>GTDDATADSRKTYTLTDYLKNTYRLKLYSLRWISDHEYLYKQENNILVFNAEYGNSSVFLENSTFDEFGHSINDYSISPDGQFILLEYNYVKQWRHSYTASYDIYDLNKRQLITEERIPNNTQWVTWSPVGHKLAYVWNNDIYVKIEPNLPSYRITWTGKEDIIYNGITDWVYEEEVFSAYSALWWSPNGTFLAYAQFNDTEVPLIEYSFYSDESLQYPKTVRVPYPKAGAVNPTVKFFVVNTDSLSSVTNATSIQITAPASMLIGDHYLCDVTWATQERISLQWLRRIQNYSVMDICDYDESSGRWNCLVARQHIEMSTTGWVGRFRPSEPHFTLDGNSFYKIISNEEGYRHICYFQIDKKDCTFITKGTWEVIGIEALTSDYLYYISNEYKGMPGGRNLYKIQLSDYTKVTCLSCELNPERCQYYSVSFSKEAKYYQLRCSGPGLPLYTLHSSVNDKGLRVLEDNSALDKMLQNVQMPSKKLDFIILNETKFWYQMILPPHFDKSKKYPLLLDVYAGPCSQKADTVFRLNWATYLASTENIIVASFDGRGSGYQGDKIMHA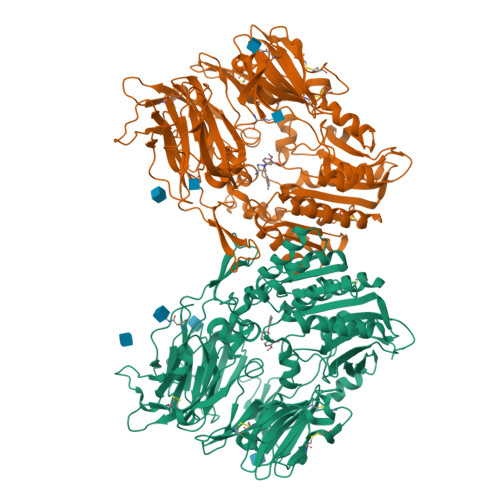INRRLGTFEVEDQIEAARQFSKMGFVDNKRIAIWGWSYGGYVTSMVLGSGSGVFKCGIAVAPVSRWEYYDSVYTERYMGLPTPEDNLDHYRNSTVMSRAENFKQVEYLLIHGTADDNVHFQQSAQISKALVDVGVDFQAMWYTDEDHGIASSTAHQHIYTHMSHFIKQCFSLP[2x]>MASHHHHHHHMSGIQTVSKSATDLTEMVKKITTMNRGEFRQITLATGAGKTTELPRSVIEEIGRHKRVLVLIPLRAAAESVYQYMRQKHPSIAFNLRIGEMKEGDMATGITYASYGYFCQMSQPKLRAAMVEYSFIFLDEYHCATPEQLAIMGKIHRFSENLRVVAMTATPAGTVTTTGQKHPIEEFIAPEVMKGEDLGSEYLDIAGLKIPVEEMKNNMLVFVPTRNMAVEAAKKLKAKGYNSGYYYSGEDPSNLRVVTSQSPYVVVATNAIESGVTLPDLDVVVDTGLKCEKRIRLSPKMPFIVTGLKRMAVTIGEQAQRRGRVGRVKPGRYYRSQETPVGSKDYHYDLLQAQRYGIEDGINITKSFREMNYDWSLYEEDSLMITQLEILNN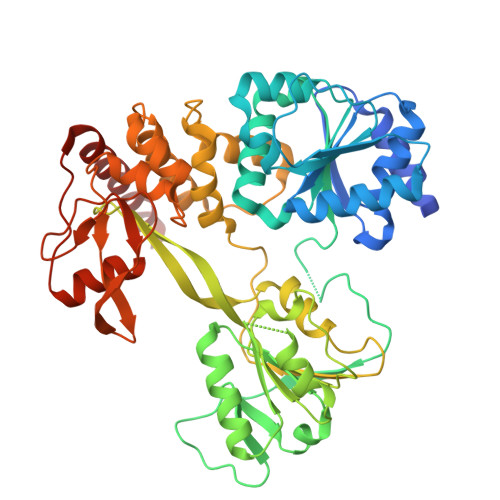LLISEELPMAVKYIMARTDHPEPIQLAYNSYETQVPVLFPKIRNGEVTDTYDNYTFLNARKLGDDVPPYVYATEDEDLAVELLGLDWPDPGNQGTVEAGRALKQVVGLSTAENALL[4x]> MSEPEVPFKVVAQFPYKSDYEDDLNFEKDQEIIVTSVEDAEWYFGEYQDS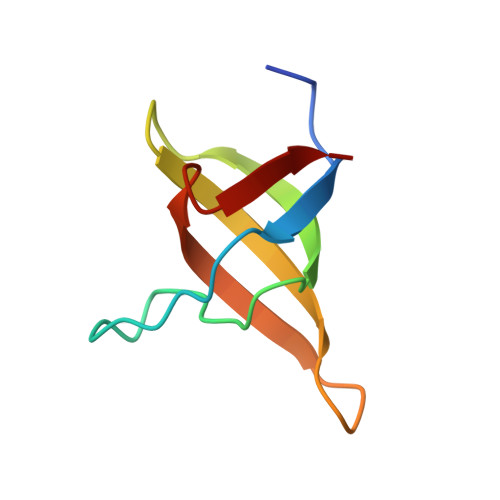NGDVIEGIFPKSFVAVQG>[12x]MAASGEPQRQWQEEVAAVVVVGSCMTDLVSLTSRLPKTGETIHGHKFFIGFGGKGANQCVQAARLGAMTSMVCKVGKDSFGNDYIENLKQNDISTEFTYQTKDAATGTASIIVNNEGQNIIVIVAGANLLLNTEDLRAAANVISRAKVMVCQLEITPATSLEALTMARRSGVKTLFNPAPAIADLDPQFYTLSDVFCCNESEAEILTGLTVGSAADAGEAALVLLKRGCQVVIITLGAEGCVVLSQTEP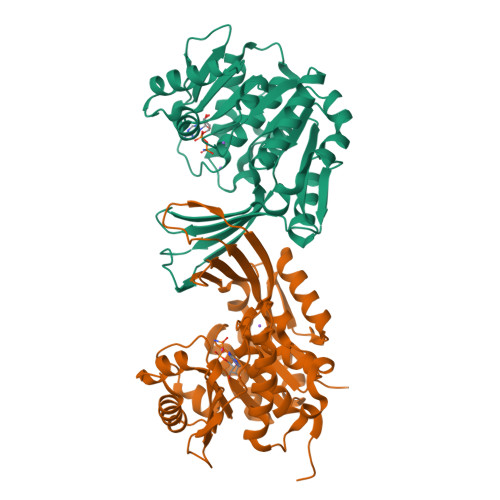EPKHIPTEKVKAVDTTGAGDSFVGALAFYLAYYPNLSLEDMLNRSNFIAAVSVQAAGTQSSYPYKKDLPLTLFLEHHHHHH>MRYAETGYVLEVDLTKGSIERVATDPRDTELYLGGLGTNAKILWDRVPPEVEPFSPENLLIFAAGLLCGTPATGCNRTIVSTVSPQTKLMAFSMMGGFWAPELKYAGYDKIIFRGKSPELVYLYINNDKVEIRDASHLKGKGAIETAEIIKKELNEPRAQVAAIGKAGENRVFYASIEQGRSSASRGGIGAVMGDKGLKAVVVRGTKDLCVAKPEEYIGLCNEVLDYIKHREENPIPDVMPILAGLGSPQEMKVHDEKWHTENFNWGNARTRRKDFWTDEVSHAWEKTMDKARTRLISCYNCPMKCGATISMEGLPTYMMKCFTKLTYTMAAYSDLDFGLRIAQKATEYGLDGFSAPQVMAFAFELLEKGILKDSDFPGLPEGNEERFFYLLDKIVNRDGIGDILANGTYWAAQEIGNGAEDYAHNNIKKHEQLPLKLSMLNPIYYLMYCTGEKINITQIEGQFPQAPYPKLEQREAFVEDWIQVPDEKFKKIFLEWEPRGEKSMPNFPTVDMCCDIVDWQEMMHYIDDALGQCAGLSSFPLKPPYHIHNYPKFIAAGAGIEMDTEKLKKAAKRYRTLVRAFNIRRGMRRVDEQPPANHWKNRFPELEKELLDSYYKLKGWNDDGIPTKETLDDLGLGYVGD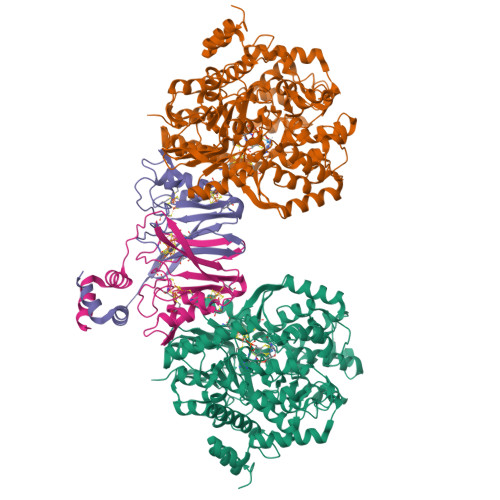EFIKRGILSAG[4x];>MNSETKKRIVKTINIDADKCNGCRACEVICSAFHAMPPYSSNNPARSRVRVVRDPLRDIYVPLYAGEYTESECIGRDKFIIDGKEYDECGFCRASCPSRDLFREPDSGLPLKCDLCDGEPEPLCVKWCLVGALSVTEREVEEPDESVKRTEMEIGLESLISRFGADVVADTVEQLTKKR[4x]N-METHYL-4-DEOXY-4-AMINO-PYRIDOXAL-5-PHOSPHATE | C9 H16 N2 O5 P | 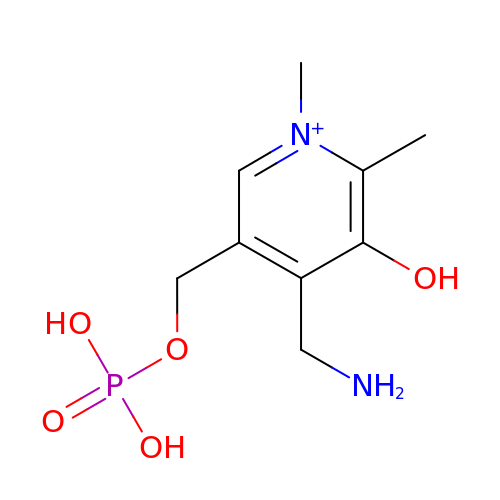BDHMQTZHNOSTBZ-UHFFFAOYSA-O2-{[1-(3,5-dimethylphenyl)-1H-imidazol-2-yl]sulfanyl}-N-hydroxyacetamide 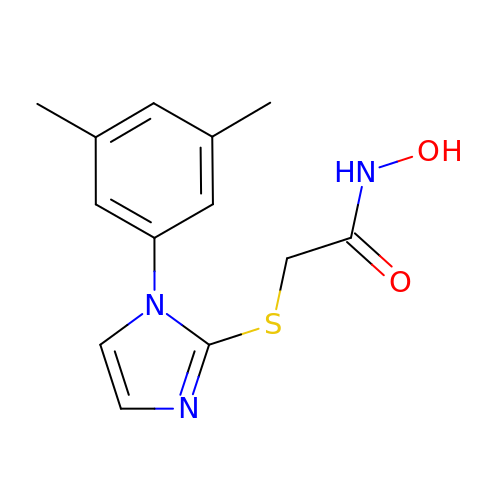| C13 H15 N3 O2 S | KKPWLEDZKPGXQJ-UHFFFAOYSA-N>LTLGNTTSSVILTNYMDTQYYGEIGIGTPPQTFKVVFDTGSSNVWVPSSKCSRLYTACVYHKLFDASDSSSYKHNGTELTLRYSTGTVSGFLSQDIITVGGITVTQMFGEVTEMPALPFMLAEFDGVVGMGFIEQAIGRVTPIFDNIISQGVLKEDVFSFYYNRDSENSQSLGGQIVLGGSDPQHYEGNFHYINLIKTGVWQIQMKGVSVGSSTLLCEDGCLALVDTGASYISGSTSSIEKLMEALGAKKRLFDYVVKCNEGPTLPDISFHLGGKEYTLTSADYVFQESYSSKKLCTLAIHAMDIPPP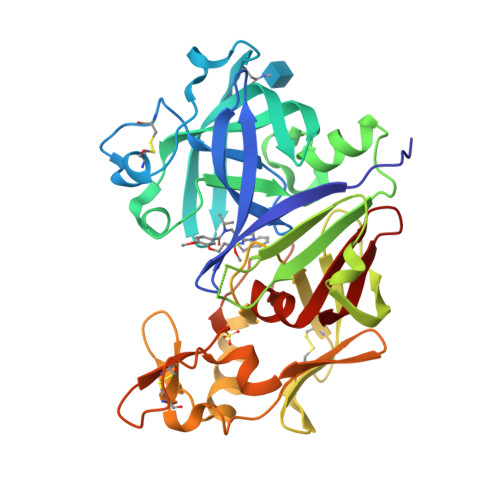TGPTWALGATFIRKFYTEFDRRNNRIGFALAR[2x]> IVLEPIYWNSSNSKFLPGQGLVLYPQIGDKLDIICPKVDSKTVGQYEYYKVYMVDKDQADRCTIKKENTPLLNCARPDQDVKFTIKFQEFSPNLWGLEFQKNKDYYIISTSNGSLEGLDNQEGGVCQTRAMKI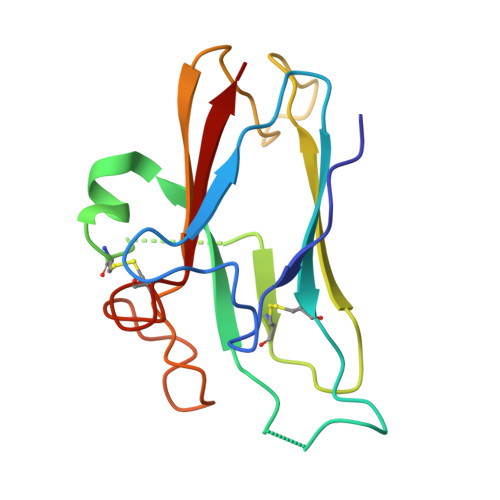LMKVG>[2x]MNITGKGAYDTGTYANLFQRSGYREDEIKARLEQTWNDLFYGDEHTRIYYPVGDDKGYMLDTGNDDVRSEGMSYGMMMAVQMDKKHEFDRLWNYAYTYMQHTEGRYKDYFAWHCKPDGTRLSPGPAPDGEEFFAMALFFASNRWGDGP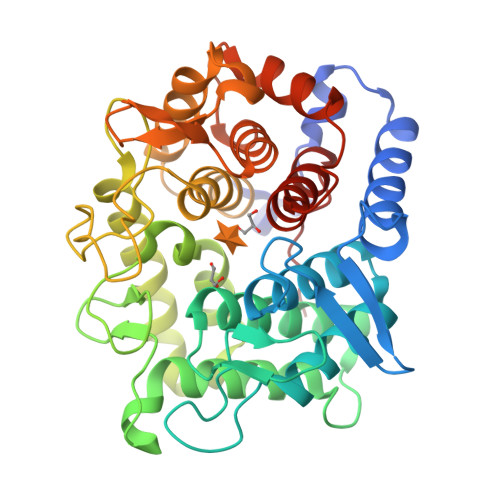APYDYQAQARKILHACLHQGEQGEGDPMWEPSNRLIKFIPELPFSDPSYHLPHFYELFAQYANEQDRTFWKEAAEASRAYLRTACHPVTGLSPEYANYDGTPAPVQLHGDFRHFYSDAYRVAANVALDWEWFRKDPWQVQQSNRIQAFFSDIDVSDYRRYTIEGEPFNEPALHPVGLLATNAMASLAADGPDADSFVKRFWNTPLRQGKRRYYDNCLYFFTMLALSGNYRVYQQ6-(but-3-en-1-yl)-4-[1-methyl-6-(morpholine-4-carbonyl)-1H-benzimidazol-4-yl]-1,6-dihydro-7H-pyrrolo[2,3-c]pyridin-7-one | C24 H25 N5 O3 | 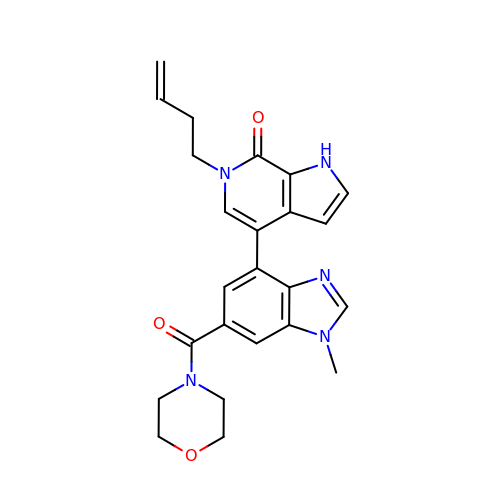XJRUWGFZGQNPPD-UHFFFAOYSA-N>ETVPLILLVPKSRREDLEKAQLAERMRSQFFIDYGVRLPEVLLRDGEGLDDNSIVLLINEIRVEQFTVYFDLMRVVNYSDEVVSFGINPTIHQQGSSQYFWVTHEEGEKLREMGYVLRNALDELYHCLAVTLARNVNEYFGIQETKHMLDQLEAKFPDLLKEV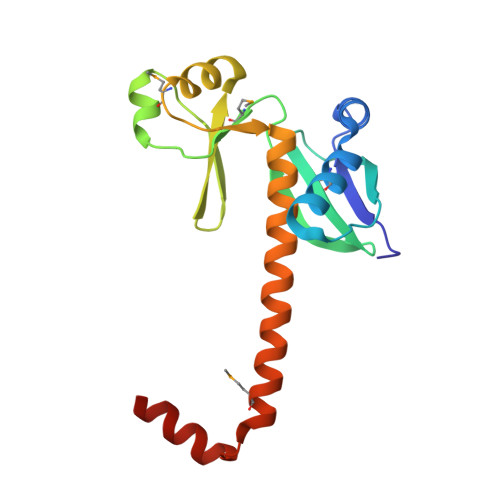LRHAT[2x]> METKLTYGNRVTLPEFAKYIVAPAFHEIEGRAIPVTGVDDDASGTQATKLPFVLVGLRQGDTSGPATIAGNSTINLRDDFIVEFNMKKERYRDRKGGETPFFSYYDYESIRDRLFNSMIEFSGEHGITFEFVSLDISTEGDVVYIEFRFRQNYEWCETVREADTTIEAGRFSIN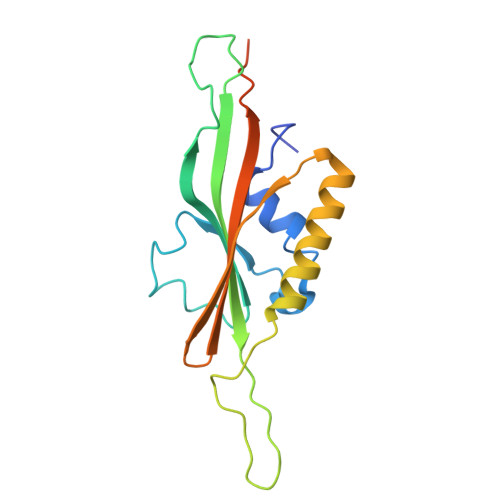LQGC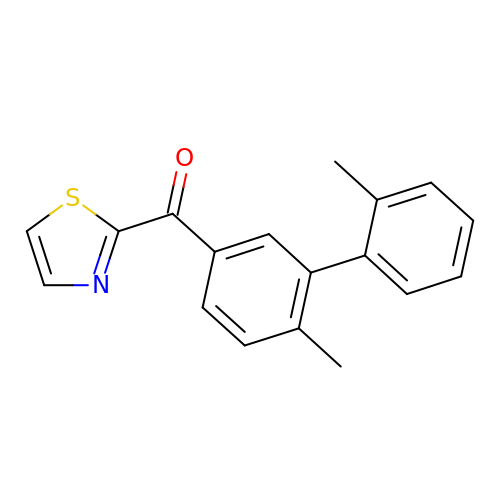(2',6-dimethyl[1,1'-biphenyl]-3-yl)(1,3-thiazol-2-yl)methanone | C18 H15 N O S | WEOQMVQEKRDUIM-UHFFFAOYSA-N>SQENTNNRSPQVGRAPRNTEVEQMTTLSNRAQEFNRRLTQKTDNAPWRRVVYRRVDLMEESNAVLYYPPRPIGDRKNLFSTIFGLINSNSLDVYEYLDGFEAFTDQYKIKFQEFLDRFGIYYQPSTNKNAELFKVADSDIPSAEVKAYYVKEEWYFT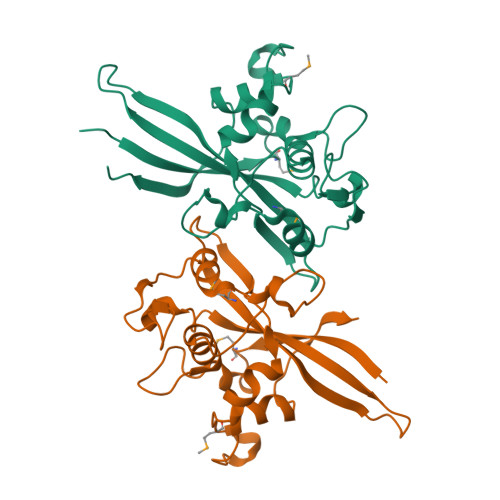PTNSDVDIKIQAICPIMTGQDEFGEVRNQPLFWIPYENIRPYIARERVMLSSLNNTRNSTIDDFFRLNLYKGDIVKTENLHNRALAE[2x]> MPSNNRYDVTEWPAGNPAKDIGEVINSIIADIKARQGAADVDDGGKPGAVIYLPPGDYHLRTQVLIDISFLRIEGSGHGFTSSSIRFNVPEEEWPDLHELWPGGSRVIVDLPAGGAGDSAAGAAFLVAREGSPRISSVEFSNFCIDGLHFTADGSGRHPENTYANGKTGIHVASANDSFRVTDMGFVYLENALTIHKADALSIHHNFIAECGSCIELRGWGQASKITDNLVGAGPRGHSIYAENHGGLLVTANNVFPRGASSVHFKGVTRSSVTNNRLHAFYPGMVRLEEN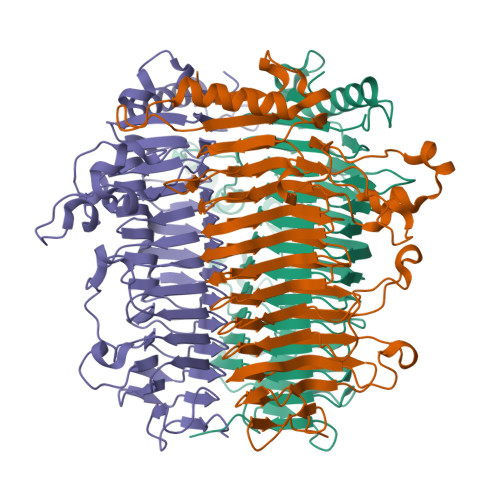SSENLVATNHFLRDHEPWTPFFGVDNGLDDLTGLLSISGNNNSVIGNHFSEVVDANEIRPEGATPVIIRLTAGTGNFVSTNHVVSNVDTQHVLVDPGSARNTILDSGSDTQVVADRAVNAIRATPTVGF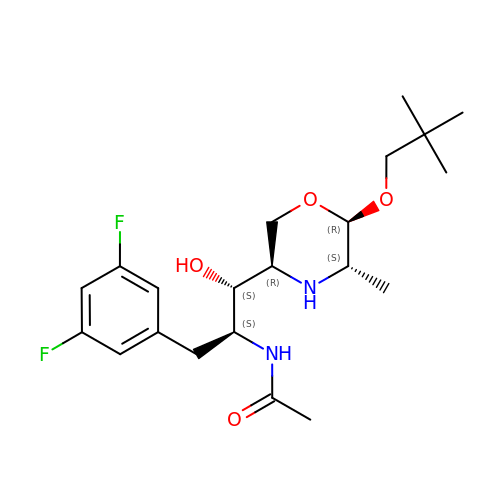N-{(1S,2S)-3-(3,5-difluorophenyl)-1-[(3R,5S,6R)-6-(2,2-dimethylpropoxy)-5-methylmorpholin-3-yl]-1-hydroxypropan-2-yl}acetamide | C21 H32 F2 N2 O4 | MTSIVXGKWLWPKB-VVEMMYRFSA-N>[2x]PISKMVTAHFVLIHTICHGAWIWHKLKPALERAGHKVTALDMAASGIDPRQIEQINSFDEYSEPLLTFLEKLPQGEKVIIVGESCAGLNIAIAADRYVDKIAAGVFHNSLLPDTVHSPSYTVEKLLESFPDARDTEYFTFTNITGETITTMKLGFVLLRENLFTKCTDGEYELAKMVMRKGSLFQNVLAQRPKFTEKGYGSIKKVYIWTDQDKIFLPDFQRWQIANYKP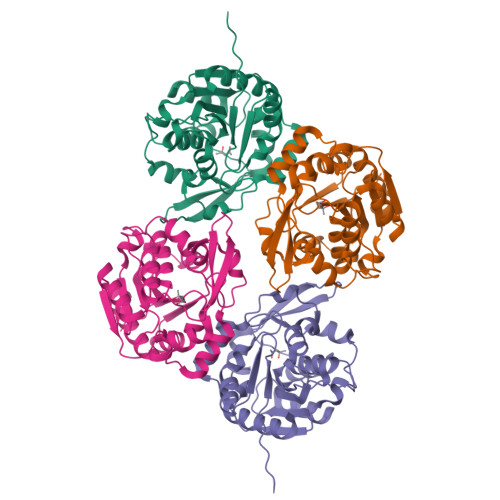DKVYQVQGGDHKLQLTKTEEVAHILQEVADAYA> QECTKFKVSSCRECIESGPGCTWCQKLNFTGPGDPDSIRCDTRPQLLMRGCAADDIMDPTSLAETQEDHNGGQKQLSPQKVTLYLRPGQAAAFNVTFRRAKGYPIDLYYLMDLSYSMLDDLRNVKKLGGDLLRALNEITESGRIGFGSFVDKTVLPFVNTHPDKLRNPCPNKEKECQPPFAFRHVLKLTNNSNQFQTEVGKQLISGNLDAPEGGLDAMMQVAACPEEIGWRKVTRLLVFATDDGFHFAGDGKLGAILTPNDGRCHLEDNLYKRSNEFDYPSVGQLAHKLAENNIQPIFAVTSRMVKTYEKLTEIIPKSAVGELSEDSSNVVQLIKNAYNKLSSRVFLDHNALPDTLKVTYDSFCSNGVTHRNQPRGDCDGVQINVPITFQVKVTATECIQEQSFVIRALGFTDIVTVQVLPQCECRCRDQSRDRSLCHGKGFLECGICRCDTGYIGKNCEP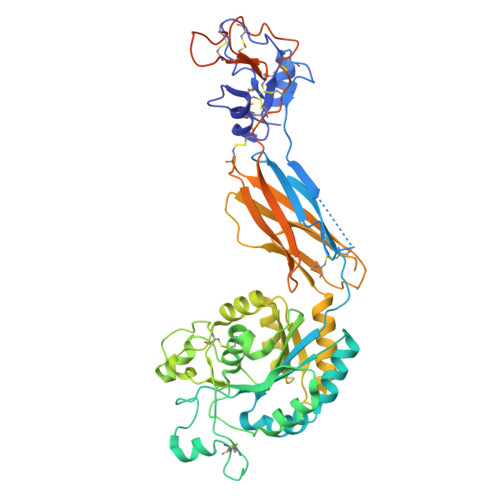AALQTLFQGPLGAQGKKKLQALKKKNAQLKWKLQALKKKLAQHHHHHHA>[2x]GHTNNTNNKGLSASINNGVGSSSSNNTYVTPQAFWNLYFDFTGDETPGYPKGKINISQTLFQSEMKKNSS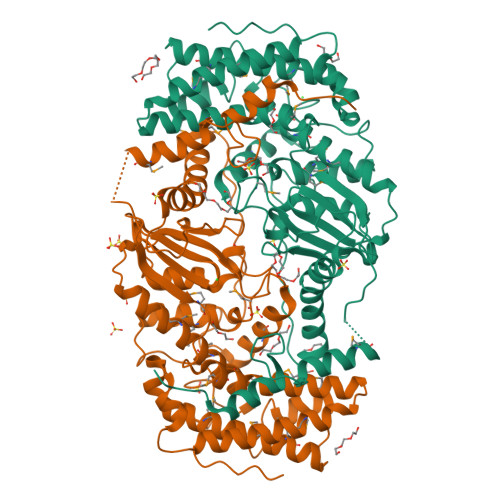LAQQNEGQLILFINSTLYIYNSDRQLKLKQLMRTAPNSGFTEMTAISHIGPALMYLAKIKENGDASWKSQMENLLKDIQAVKVINAQTPNNWLEQVNAPAWKPHLTTIHNMIDYACSMAGNYMSDVLNEKLSFDMASLQNDFLNGNKTYPIPYNNVMIGTFMLTALQSMDQLHSKISQLKIDWPHAKVIIRFVAGSNVSAGVSKGSNWLVPFVQALSNNKLATDRIYITPYAAVKPSLGAQELTQADYNYYNNTVWGARHNRRIIANEVFTNITSIFLPDRPAIPGDYTYSKPPKIEDFLMRLKFSLAEPTEMLSNTVGFWMAGELAEKNWNYNKISIPGITTGFPEGISTYPNNNPVIQR> MGHWTLSGILAFLL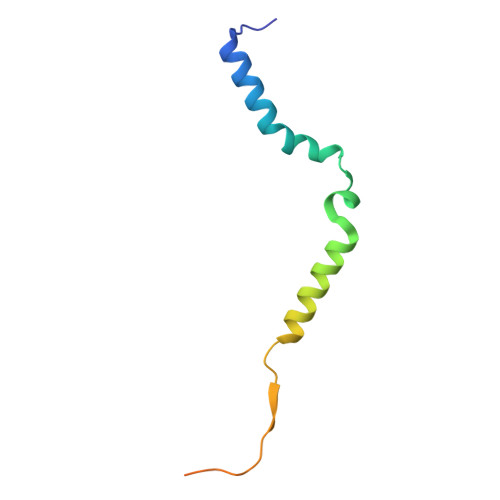LLSLLLPSLLIMFIPLTFRRPASSWKARSLQKILLMASSVRLKPLSSSRIPCVLRPDSKRRFHHHHHH> GPLQEEDTFRELRIFLRNVTHRLAIDKRFRVFTKPVDPDEV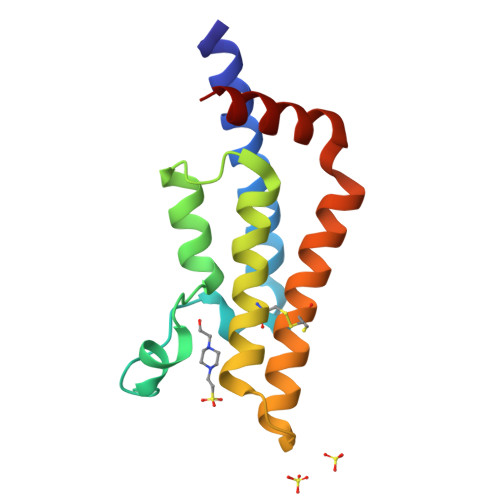PDYVTVIKQPMDLSSVISKIDLHKYLTVKDYLRDIDLICSNALEYNPDRDPGDRLIRHRACALRDTAYAIIKEELDEDFEQLCEEIQESR>GAMEMNMA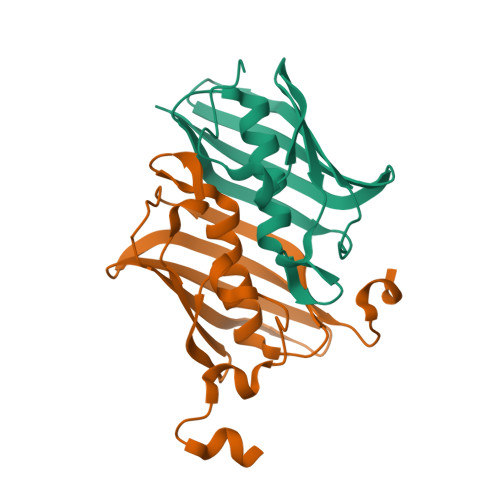DAPLEEGLLVCTRLDQNLCAELISFGSGKATVCLTPKEFMLAEDDVVHAGFIVGAASFAALCALNKKNSLISSMKVNLLAPIEIKQEIYFNATITHTSSKKSTIRVEGEFMEIKVFEGDFEILVFEKRPFKFNFKED[2x]>[12x]MSKPVKIGPWGGNGGSERDVQPKPIRMVSMTVSSGAIVDAIAFTYVGTDNVQHSSGIKWGGTGGTEDTINLDATNYVTEISGTVGKFGTDDIVT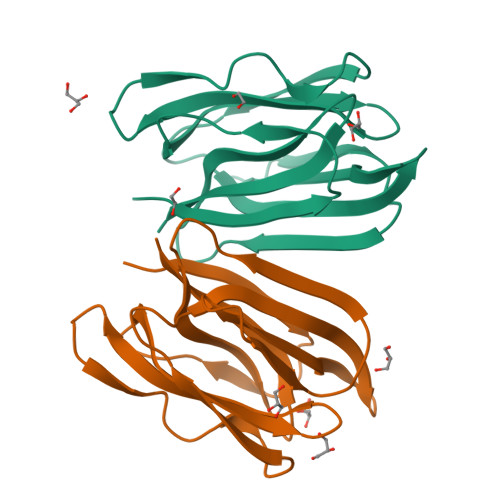SLKIITSKGVTRTYGSGTGIPFRVPVLDGGKIAGFFGRAGAFLDAIGFYITP Porphyromonas gingivalis is a major pathogenic oral bacterium that is responsible for periodontal disease. P. gingivalis exerts its pathogenic effects through mechanisms such as immune evasion and tissue destruction, primarily by secreting various factors, including cysteine proteases such as gingipain K (Kgp), gingipain R (RgpA and RgpB) and PrtH (UniProtKB ID P46071). Although its detailed function has not been elucidated, PrtH contains 989 amino-acid residues and multiple domains, including a cleaved adhesion domain, small Ig-like fold domains and a DUF2436 domain. Although the structure and function of the catalytic domain and some K domains of gingipains are known, the structure and function of DUF2436 have not been characterized.

We recombinantly expressed the DUF2436 domain (residues Ser361–Cys579) of PrtH (UniProtKB ID P46071) from P. gingivalis in Escherichia coli. Purified recombinant PgDUF2436 was successfully crystallized by the sitting-drop vapor-diffusion method at 293 K. The crystal belonged to space group P3221 and contained a monomer of PgDUF2436 in the asymmetric unit. In this study, the DUF2436 domain of PrtH from P. gingivalis (PgDUF2436) was determined at 2.21 Å resolution, revealing a noncanonical β-jelly-roll sandwich topology with two antiparallel β-sheets and one short α-helix. Met516–Cys579 were not modeled in this structure because of very weak electron density in this region. The size-exclusion chromatography result indicated that PgDUF2436 exists as a monomer in solution. Analysis of the electrostatic surface charge of the PgDUF2436 structure reveals the presence and location of negatively charged patches. The negatively charged patch on β3, β5, β8 and β9 is formed by Asp407, Asp409, Asp431, Asp446, Glu438, Asp497 and Asp498. Although the structure of PgDUF2436 was determined by the molecular-replacement method using an AlphaFold model structure as a template, there were significant differences in the positions of β1 between the AlphaFold model and the experimentally determined PgDUF2436 structure. However, DaliLite search results using structure-based alignment revealed that the PgDUF2436 structure has structural similarity Z-scores of 5.9–5.4 with the C-terminal domain of AlgF, the D4 domain of cytolysin, IglE and the extracellular domain structure of PepT2. Collectively, these results demonstrate that PgDUF2436 exhibits a novel structure with a modified β-jelly-roll sandwich fold topology.

> MSREVKRIGDGLFVTIEPANDVRANEAKVVLAADNVWGDNTGYQFLLDADHNTFGSVIPATGPLFTGTASSDLYSANFEYLIPANADPVVTTQNIIVTGQGEVVIPGGVYDYCITNPEPASGKMWIAGDGGNQPARYDDFTFEAGKKYTFTMRRAGMGDGTDMEVEDDSPASYTYTVYRDGTKIKEGLTETTYRDAGLSAQSHEYCVEVKYTAGVSPKVC>GSHMNIITVTLNMEKYNFLGISIVGQSNERGDGGIYIGSIMKGGAVAADGRIEPGDMLLQVNDMNFENMSNDDAVRVLRDIV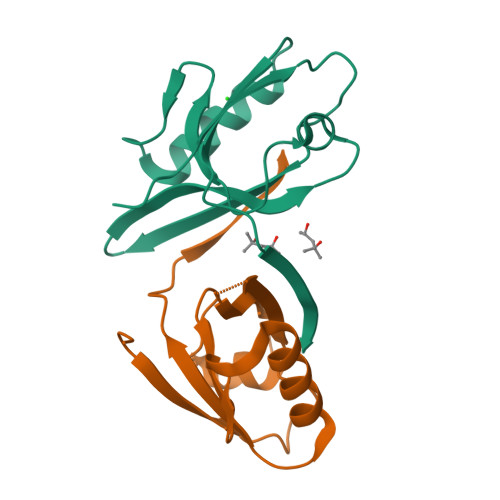HKPGPIVLTVAKSGGGWKWYGWF[2x]>[2x]MIVFTDLDGTLLDERGELGPAREALERLRALGVPVVPVTAKTRKEVEALGLEPPFIVENGGGLYLPRDWPVRAGRPKGGYRVVSLAWPYRKVRARLREAEALAGRPILGYGDLTAEAVARLTGLSREAARRAKAREYDETLVLCPEEVEAVLEALEAVGLEWTHGGRFYHAAKGADKGRAVARLRALWPDPEEARFAVGLGDSLNDLPLFRAVDLAVYVGRGDPPEG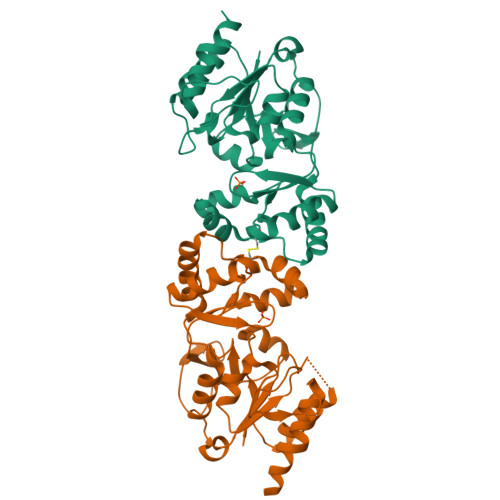VLATPAPGPEGFRYAVERYLLPRLSRRGGSGP>[6x]HHHHHHENLYFGMAEFDAVTAFADAPAAVLSTLNADGAPHLVPVVFAVHVPHVEGQPARIYTAVDAKRKTTRNLRRLANIDRDSRVSLLVDHYS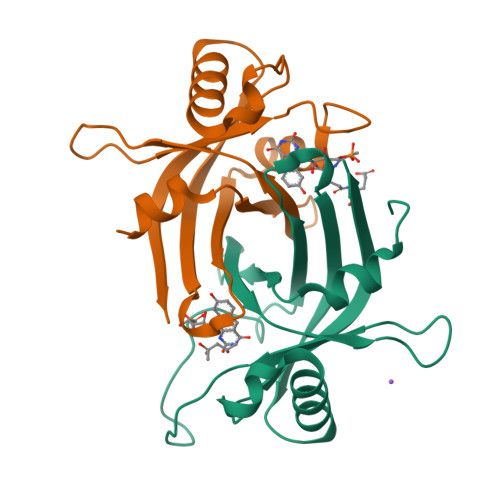DDWTQLWWVRADGVATTHHSGDEVATGYALLRAKYHQYERVSLDGPVISVEVSRWASWQA> AYQ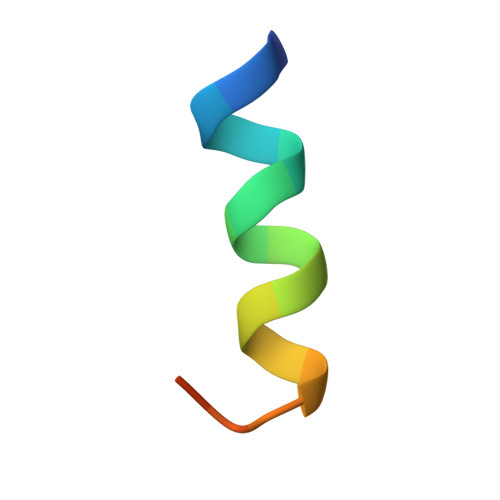QGQNQLYNELNLGRR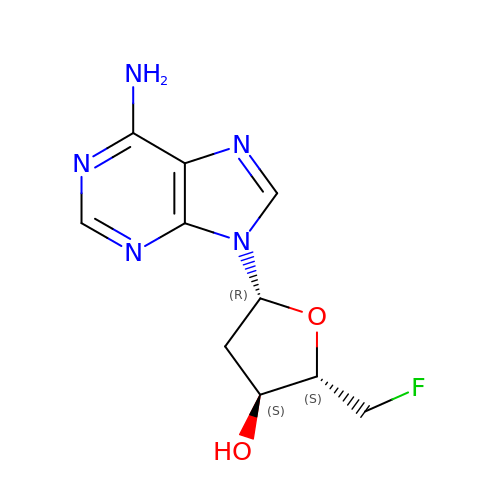5'-FLUORO-2',5'-DIDEOXYADENOSINE | C10 H12 F N5 O2 | QKUCDAPGYBWICH-RRKCRQDMSA-N> GSHMPPPDPAAMGTWKFFRASVDGRPVFKKEFDKLPDQARAALIVLMQRYLVGDLAAGSIKPIRGDILELRWHEANNHFRVLFFRWGQHPVALTAFYANQQKTPKTKIETALDRQKIWKRAFGDTPPILE

Here, we focus on the deleterious toxin of the atypical tripartite toxin-antitoxin-chaperone (TAC) system of Mycobacterium tuberculosis, whose inhibition requires the concerted action of the antitoxin and its dedicated SecB-like chaperone. In addition, we show that HigBTAC functions as a bona fide RNase that specifically cleaves mRNA after the second nucleotide of A-site codons (mainly CCA codons) during translation. HigBTAC has a similar compact fold as other RelE homologs, with four antiparallel β-strands flanked by three α-helices.

In addition, alanine substitution of residue K95 of HigBTAC, which possibly corresponds to the active site residue R81 of E. coli RelE29, fully inhibited toxicity in vivo in M. smegmatis. Note that the K95A substitution that leads to the inactive toxin was used as non-toxic HigBTAC control for further in vivo and in vitro analysis. In parallel, the crystal structure of isolated monomeric HigBTAC[K95A] was obtained at a 1.9 Å resolution and used to compare possible conformational changes that may occur upon association with the ribosome. Notably, these regions include most of the proposed catalytic residues of HigBTAC (i.e., E66, R68, N73, K95, F93, Q98, and K99), suggesting that such differences could have some functional significance. In support of this, the structure of HigBTAC clearly differs from the alpha-fold models of HigB2 and HigB3 in particular in the two loops between β2-β3 and β4-α3, which contain most of the catalytic residues.>[5x]GAMAWPEESEKRKRVSSAVQFL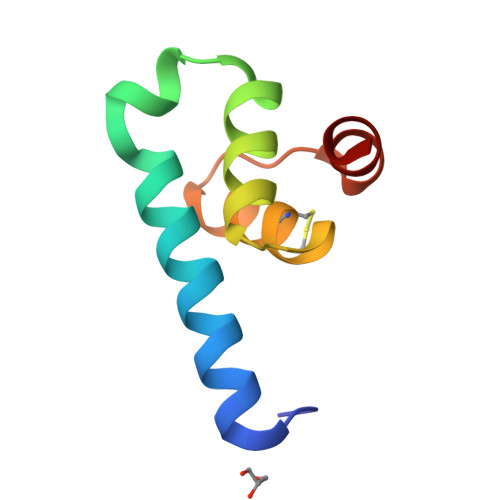HDSRVKITPAANKIQFLKSKGLTTEEVCEAFEKAGQTIPLDEIKKIMN>[2x]MNQLNTAIVEKEVIDPMAFRRALGNFATGVTIMTAQTSSGERVGVTANSFN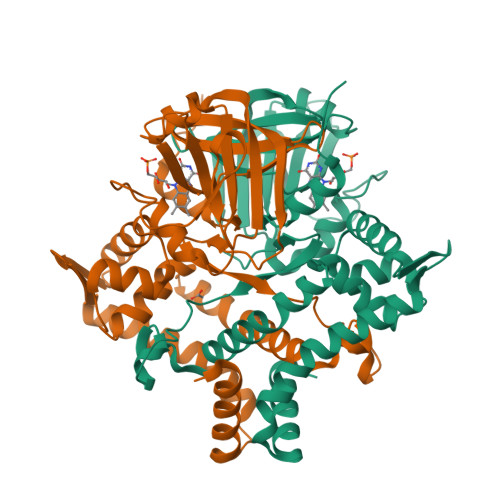SVSLDPALVLWSIDKKSSSYRIFEEATHFGVNILSAAQIELSNRFARRSEDKFANIEFDLGVGNIPLFKNCSAAFECERYNIVEGGDHWIIIGRVVKFHDHGRSPLLYHQGAYSAVLPHPSLNMKSETAEGVFPGRLYDNMYYLLTQAVRAYQNDYQPKQLASGFRTSEARLLLVLESKTASSKCDLQREVAMPIREIEEATKILSEKGLLIDNGQHYELTEQGNACAHMLYKIAESHQEEVFAKYTVDERKLFKNMLKDLIGI6-METHYL-2(PROPANE-1-SULFONYL)-2H-THIENO[3,2-D][1,2,3]DIAZABORININ-1-OL | 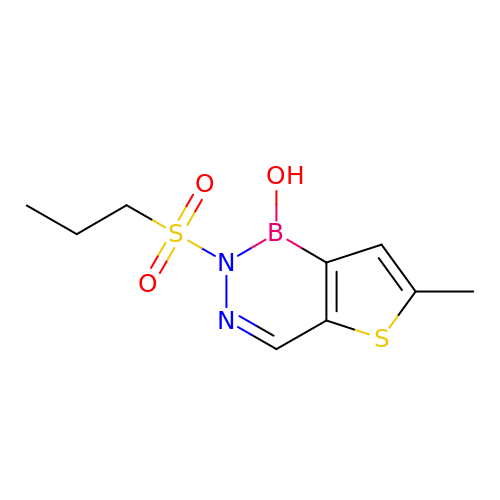C9 H13 B N2 O3 S2 | TVXLILKNSPCVRB-UHFFFAOYSA-N Left-handed duplexes of Z-DNA with the self-complementary d(CGCGCG) sequence are remarkable for their potential to form crystals that diffract X-rays to very high resolution. The asymmetric unit of the complex contains one d(CGCGCG)2 Z-DNA duplex. The general structural parameters of the DNA double helix in the complex classify it into the Z-DNA family of duplexes.

In the present study, using high-resolution crystallographic data, we describe the coordination geometry of three hydrated Cr3+ ions and their outer-sphere interactions with a highly disordered Z-DNA chain in a d(CGCGCG)2–Cr3+ complex. The high-resolution crystal structure of the d(CGCGCG)2–Cr3+ complex presented in this work shows the presence of three Cr3+ ion sites per one Z-DNA duplex, which do not form any direct coordination bonds with either the guanine N/O atoms or the phosphate groups of the DNA. Only water-mediated contacts between the nucleic acid and the Cr3+ cations are observed. The Cr3+(1), Cr3+(2) and Cr3+(3) ions have partial occupancies of 35, 26 and 40 %, respectively. The Cr3+(1) and Cr3+(2) ions are bridged by three water molecules from their coordination spheres, one of which (Wat1) is split into two sites. The coordination sphere of Cr3+(3) is square pyramidal, with five water molecules, one of which (Wat37) is split into two sites. A characteristic feature of the d(CGCGCG)2–Cr3+ structure is a high degree of disorder of the DNA chains. In addition, the electron density map clearly shows alternative positions for both the base and deoxyribose rings of the G2 nucleotide. The ZII conformations are stabilized by hydrogen bonds between a phosphate oxygen atom and water molecules form the coordination spheres of the Cr3+ cations, as well as by contacts with symmetry-related Z-DNA helices in the crystal lattice. The d(CGCGCG)2–Cr3+ structure is an excellent illustration of the flexibility of the Z-DNA molecule, visible in the adoption of multiple conformations (by the phosphate groups and the G2 nucleotide), in response to changes in its electrostatic and hydration environment, caused by the introduction of hydrated metal complexes.

>CGCGCG[2x]GpsB has emerged as a major regulator of PG biosynthesis in low G+C Gram-positive bacteria, and its homologues (DivIVA/Wag31/antigen 84) in Actinobacteria play essential roles in hyphal growth and branching. To gain molecular understanding of GpsB function, we report three crystal structures of PBP cytoplasmic mini-domains in complex with GpsB, the first structures of a PG synthase in complex with a cytoplasmic cell cycle regulator. The PG synthase arginine finger pokes into a negatively charged cavity situated between α-helices 1 and 2 of GpsB and is fixed in the same orientation in all structures, just as the phosphoryl group defines the binding orientation of peptides to 14-3-345. Therefore, the role of GpsB in the bacterial cell cycle is that of an adaptor, docking PG synthases to other cell wall enzymes, scaffolds and shape determinants into protein complexes for division (the divisome) and peripheral growth (the elongasome).

S. pneumoniae, more distantly related to either Bacillus or Listeria, is an ovoid-shaped Gram-positive coccus in which GpsB is essential. In S. pneumoniae, GpsB localises to mid-cell, the only region of active PG synthesis for both peripheral (side-wall) elongation and cell division in this bacterium. SpGpsB co-immunoprecipitated with SpPBP2a (one of three pneumococcal class A PBPs), SpMreC and other proteins, suggesting they interact at some point in the pneumococcal cell cycle. The importance of the SpGpsB residues involved in the interactions with SpPBP2a is also consistent with the phenotype because of the severe growth and morphological defects of S. pneumoniae strains harbouring the SpGpsBTyr23Ala, SpGpsBVal28Ala, SpGpsBAsp29Ala, SpGpsBLeu32Ala and SpGpsBAsp33Ala alleles even though the mutated proteins were still capable of self-interactions and were expressed at wild-type levels. SpGpsBTyr23Ala and SpGpsBAsp29Ala mutations had a greater impact on SpMreC interactions than SpGpsBAsp33Ala; this pattern mirrors the impact of the equivalent mutations (LmGpsBTyr27Ala, LmGpsBAsp33Ala and LmGpsBAsp37Ala) on MreC interactions in L. monocytogenes and thus substantiates the evidence that different surfaces are used by GpsB to bind a specific class A PBP and MreC. Whilst the interactions of SpGpsB with SpEzrA and SpStkP were confirmed by BACTH, and observed with the reciprocal hybrid pairs, they were unaffected by any of the SpGpsB alleles mentioned above.

>[4x]GAIIFSAKDIFEQEFGREVRGYNKVEVDEFLDDVIKDYETYAALVKSLRQEIADLKEELTRK3-(1H-INDOL-3-YL)-4-{1-[2-(1-METHYLPYRROLIDIN-2-YL)ETHYL]-1H-INDOL-3-YL}-1H-PYRROLE-2,5-DIONE | C27 H26 N4 O2 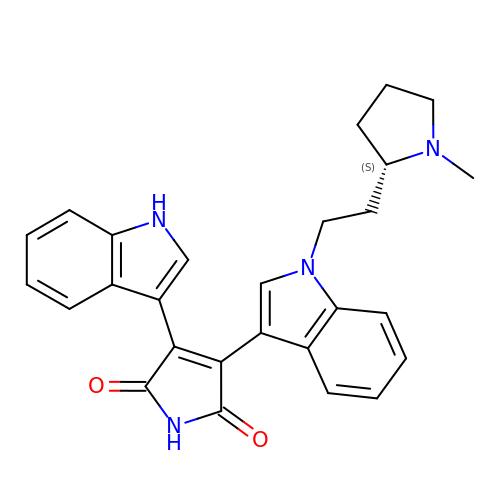| LBFDERUQORUFIN-KRWDZBQOSA-N The N-oligosaccharyl transfer is catalyzed by an integral membrane enzyme, oligosaccharyltransferase (OST). Oligosaccharyltransferase (OST) catalyzes oligosaccharide transfer to the Asn residue in the N-glycosylation sequon, Asn-X-Ser/Thr, where Pro is strictly excluded at position X. Considering the unique structural properties of proline, this exclusion may not be surprising, but the structural basis for the rejection of Pro residues should be explained explicitly. The archaeal and eubacterial OSTs are also single-subunit enzymes. The N-terminal transmembrane (TM) region of the Stt3/AglB/PglB proteins consists of 13 TM helices and contains two DXD motifs on the first and second external loops (EL1 and EL2) and a TIXE/SVSE motif on the fifth external loop (EL5).

Here, we determined the crystal structure of the ternary complex of the A. fulgidus AglB protein (AfAglB) with a sequon peptide and a dolichol-phosphate molecule. To stop the transfer reaction, the Asn residue in the sequon was replaced by a L-2,4-diaminobutyrate (Dab) residue. The acceptor peptide was tethered to the AfAglB protein via an engineered disulfide bond. Even though the tethered peptide contained the non-reactive Dab residue at position 0, the LLO binding site was occupied by a dolichol-phosphate, instead of an intact LLO, suggesting that the LLO was hydrolyzed during the prolonged crystallization period. The N-terminal half (residues 335-350) of the EL5 loop is disordered when the LLO binding site is vacant and becomes ordered to form an α-helix in the presence of dolichol-phosphate. The carboxylate group of Glu360 in the TIXE motif (Thr-Ile-Ala-Glu) indirectly participates in the coordination to the metal ion through two of the three water molecules. The sequon part, Dab-Val-Thr, plus the Ala residue at position +3 in the acceptor peptide, adopts an extended conformation and lies side-by-side in an antiparallel manner with the 4-residue TIXE motif, Thr-Ile-Ala-Glu, in the C-terminal half of the EL5 loop. Two inter-chain hydrogen bonds are formed between the carbonyl oxygen of Thr357 and the amide group of Ala+3, and between the carbonyl oxygen of Val+1 and the amide group of Ala359. All residues in the sequon sequence and the TIXE motif have ϕ values in the range from −60° to −120°, except for Val+1 in the sequon, which has a high ϕ value around −150°. The rigid ring structure of the side chain does not allow Pro to adopt such a high ϕ value and thereby excludes Pro from position +1 in the N-glycosylation sequon.

> MQNAESWFKKYWHLSVLVIAALISVKLRILNPWNSVFTWTVRLGGNDPWYYYRLIENTIHNFPHRIWFDPFTYYPYGSYTHFGPFLVYLGSIAGIIFSATSGESLRAVLAFIPAIGGVLAILPVYLLTREVFDKRAAVIAAFLIAIVPGQFLQRSILGFNDHHIWEAFWQVSALGTFLLAYNRWKGHDLSHNLTARQMAYPVIAGITIGLYVLSWGAGFIIAPIILAFMFFAFVLAGFVNADRKNLSLVAVVTFAVSALIYLPFAFNYPGFSTIFYSPFQLLVLLGSAVIAAAFYQIEKWNDVGFFERVGLGRKGMPLAVIVLTALIMGLFFVISPDFARNLLSVVRVVQPKGGALTIAEVYPFFFTHNGEFTLTNAVLHFGALFFFGMAGILYSAYRFLKRRSFPEMALLIWAIAMFIALWGQNRFAYYFAAVSAVYSALALSVVFDKLHLYRALENAIGARNKLSYFRVAFALLIALAAIYPTYILADAQSSYAGGPNKQWYDALTWMRENTPDGEKYDEYYLQLYPTPQSNKEPFSYPFETYGVISWWDYGHWIEAVAHRMPIANPFQAGIGNKYNNVPGASSFFTAENESYAEFVAEKLNVKYVVSDIEMETCKYYAMAVWAEGDLPLAEKYYGGYFYYSPTGTFGYANSQWDIPLNSIIIPLRIPSELYYSTMEAKLHLFDGSGLSHYRMIYESDYPAEWKSYSSQVNLNNESQVLQTALYEAVMRARYGVSPTMGTQEVLYKYAYTQLYEKKMGIPVKIAPSGYVKIFERVKGAVVTGKVSANVTEVSVNATIKTNQNRTFEYWQTVEVKNGTYTVVLPYSHNSDYPVKPITPYHIKAGNVVKEITIYESQVQNGEIIQLDLELALVPR;> APYAVTASCR> AVKYYTLEEIQKHNNSKSTWLILHYKVYDLTKFLEEHPGGEEELREQAGGDATENFEDVGHSTDARELSKTFIIGELHP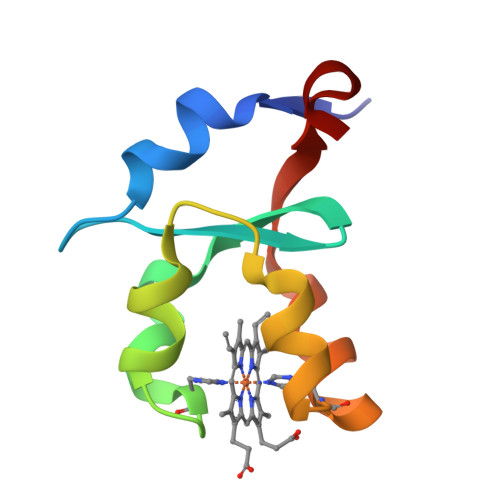DDR>TEKKYIVALDQGTTSSRAVVMDHDANIISVSQREFEQIYPKPGWVEHDPMEIWATQSSTLVEVLAKADISSDQIAAIGITNQRETTIVWEKETGKPIYNAIVWQCRRTAEICEHLKRDGLEDYIRSNTGLVIDPY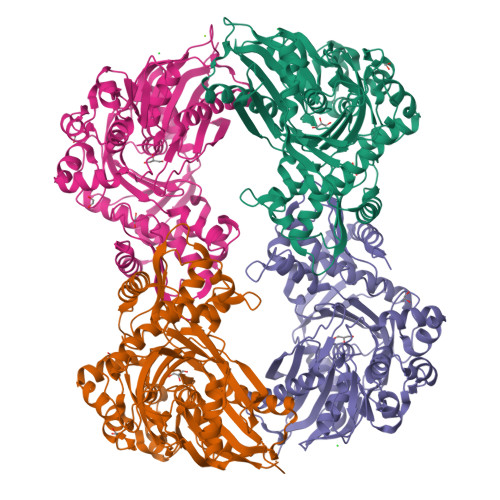FSGTKVKWILDHVEGSRERARRGELLFGTVDTWLIWKMTQGRVHVTDYTNASRTMLFNIHTLDWDDKMLEVLDIPREMLPEVRRSSEVYGQTNIDGKGGTRIPISGIAGDQQAALFGQLCVKEGMAKNTYGTGCFMLMNTGEKAVKSENGLLTTIACGPTGEVNYALEGAVFMAGASIQWLRDEMKLINDAYDSEYFATKVQNTNGVYVVPAFTGLGAPYWDPYARGAIFGLTRGVNANHIIRATLESIAYQTRDVLEAMQADSGIRLHALRVDGGAVANNFLMQFQSDILGTRVERPEVREVTALGAAYLAGLAVGFWQNLDELQEKAVIEREFRPGIETTERNYRYAGWKKAVKRAMAWEEHDQLYTRASQPELAPEDPEDLEHHHHHH[8x]> SVDVTLMPIDCELSSWSSWTTCDPCQKKRYRYAYLLQPSQFHGEPCNFSDKEVEDCVTNRPCRSQVRCEGFVCAQTGRCVNRRLLCNGDNDCGDQSDEANCRRIYKKCQHEMDQYWGIGSLASGINLFTN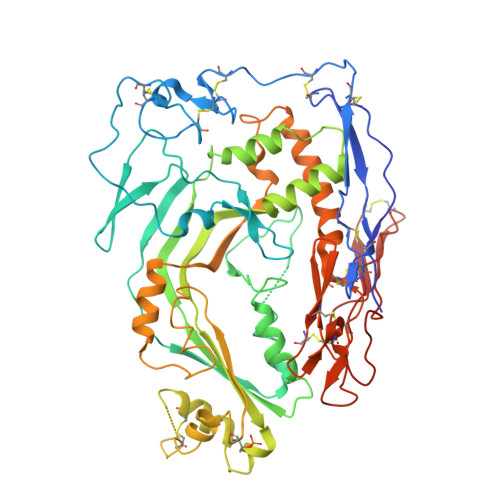SFEGPVLDHRYYAGGCSPHYILNTRFRKPYNVESYTPQTQGKYEFILKEYESYSDFERNVTEKMASKSGFSFGFKIPGIFELGISSQSDRGKHYIRRTKRFSHTKSVFLHARSDLEVAHYKLKPRSLMLHYEFLQRVKRLPLEYSYGEYRDLFRDFGTHYITEAVLGGIYEYTLVMNKEAMERGDYTLNNVHACAKNDFKIGGAIEEVYVSLGVSVGKCRGILNEIKDRNKRDTMVEDLVVLVRGGASEHITTLAYQELPTADLMQEWGDAVQYNPAIIKVKVEPLYELVTATDFAYSSTVRQNMKQALEEFQKEVSSCHCAPCQGNGVPVLKGSRCDCICPVGSQGLACEVSYRKNTPIDGKWNCWSNWSSCSGRRKTRQRQCNNPPPQNGGSPCSGPASETLDCS>MSDYGFANIEEAKADAIFKLNAQYHQDEDPKKVNMSVGAYRDDTGKPWILPAVKKASKIVEEQASFNHEYLPIAGLPRFTKAAAEVLFRPNPHLLSEDRVASMQSVSGTGANFLAASFIETFYVKHTGAHVYISNPTWPVHRTLWEKLGVTVETYPYWDAKNRSFDYEGMLSTIKSAPEGSIFLLHACAHNPTGIDPTREQWLSIFESLLSRKHLVVFDIAYQGFASGDLNRDSWALNEFVK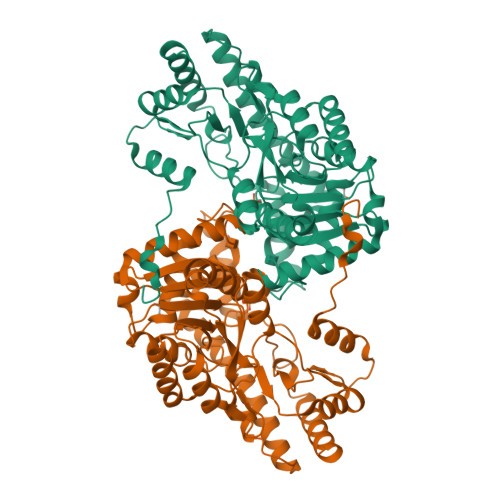YNKDFFVCQSFAKNMGLYGERTGCMHYVAKDASTKNKVLSQLCIVQRNTISNPPAYGARIAAEILNSPQLFAEWEQDLKTMSSRIIEMRKRLRDSLVALKTPGSWDHITQQIGMFSFTGLTPAQVQFCQERYHLYFSANGRISMAGLNNSNVEHVAQAFNHAVRELPLEHHHHHH[2x]>QRTGRSALAVLIRACYRLQQQLQRTRRALLHHSDAVLTSLHHVRMLL[2x];>IPAGIIPTGNVLSTIEVCIFFCIFDFFKQIRSDDNSLYSAQFDILLGTYCNTLNFVRFLELGLSVACICTKFPELAYVRDGVIQFEVQQPMIARDGPHPVDQPVHNYMVKRIHKRSLSAAFAIASEALSLLSNTYVAATEIDSSLRIRAIQQMARNLRTVSDSFERGTADQLLGVLLEKAPPLSLLSPINKFQPEGHLNRVARAALLSDLKRRVCADMFFMTRHAREPRLISAYLSDMVSCTQPSVMVSRITHTNTRGRQVDGVLVTTATLKRQLLQGILQIDDTAADVPVTYGEMVLQGTNLVTALVMGKAVRGMDDVARHLLDITDPNTLNIPSIPPQSNSDSTTAGLPVNARVPADLVIVGDKLVFLEALERRVYQATRVAYPLIGNIDITFIMPMGVFQANSMDRYTRHAGDFSTVSEQDPRQFPPQGIFFYNKDGILTQLTLRDAMGTICHSSLLDVEATLVALRQQHLDRQCYFGVYVAEGTEDTLDVQMGRFMETWADMMPHHPHWVNEHLTILQFIAPSNPRLRFELNPAFDFFVAPGDVDLPGPQRPPEAMPTVNATLRIINGNIPVPLCPISFRDCRGTQLGLGRHTMTPATIKAVKDTFEDRAYPTIFYMLEAVIHGNERNFCALLRLLTQCIRGYWEQSHRVAFVNNFHMLMYITTYLGNGELPEVCINIYRDLLQHVRALRQTITDFTIQGEGHNGETSEALNNILTDDTFIAPILWDCDALIYRDEAARDRLPAIRVSGRNGYQALHFVDMAGHNFQRRDNVLIHGRPVRGDTGQAIPITPHHDREWGILSKIYYYIVIPAFSRGSCCTMGVRYDRLYPALQAVIVPEIPADEEAPTTPEDPRHPLHAHQLVPNSLNVYFHNAHLTVDGDALLTLQELMGDMAERTTAILVSSAPDAGAATATTRNMRIYDGALYHGLIMMAYQAYDETIATGTFFYPVPVNPLFACPEHLASLRGMTNARRVLAKMVPPIPPFLGANHHATIRQPVAYHVTHSKSDFNTLTYSLLGGYFKFTPISLTHQLRTGFHPGIAFTVVRQDRFATEQLLYAERASESYFVGQIQVHHHDAIGGVNFTLTQPRAHVDLGVGYTAVCATAALRCPLTDMGNTAQNLFFSRGGVPMLHDNVTESLRRITASGGRLNPTEPLPIFGGLRPATSAGIARGQASVCEFVAMPVSTDLQYFRTACNPRGRASGMLYMGDRDADIEAIMFDHTQSDVAYTDRATLNPWASQKHSYGDRLYNGTYNLTGASPIYSPCFKFFTPAEVNTNCNTLDRLLMEAKAVASQSSTDTEYQFKRPPGSTEMTQDPCGLFQEAYPPLCSSDAAMLRTAHAGETGADEVHLAQYLIRDASPLRGCLPL[5x];> AMPFEIEVLLPGELSPAETSALQKCEGKIITFSTLRHRASLVDIALSSYYINGAPPDTLSLLEAYRMRFAAVITRVIPGKLLAHAIGVGTPTPGLFIQNTSPVDLCNGDYICLLPPVYGSADSIRLDSVGLEIVFPLTIPQTLMREIIAKVVARAVEDLNLMFSINEGCLLILALIPRLLALLIPRLLALVTREAAQLIHPEAPMLMLPIYETISSWISTSSRLGDTLGTRAILRVCVFDGPSTVHPGDRTAVIQV;> AMPFEIEVLLPGEISPAETSALQKCEGKIITFSTLRHRASLVDIALSSYYINGAPPDTLSLLEAYRMRFAAVITRVIPGKLLAHAIGVGTPTPGLFIQNTSPVDLCNGDYICLLPPVFGSADEIRLDSVGLEIVFPLTIPQTLMREIIAKVVARAVERTAADVICYNGRRYELETNLQHRDGSDAAIRTLVLNLMFSINEGTTLILTLITRLLRFPIYEAISSWISTSSRLGDTLGTRAILRVCVFDGPSTVHPGDRTAVIQV;> FKSTTQLIQQVSLTDFFRPDIEHAGSTVLILRHPTDLPALARHRAPPGRQTERLAEAWGQLLEASRAYVTSLSFIAACRAEEYTDKQAAEANRTAIVSAYGCSRMGARLIRFSECLRAMVQCHVFPHRFISFFGSLLEYTIQDNLCNITAVAKGPQEAARTDKTSTRRVTANIPACVFWDVDKDLHLSADGLKHVFLVFVYTQRRQREGVRLHLALSQLNEQCFGRGIGFLLGARICMYAAYTLIGTIPSESVRYTRRMERFGGYNVPTIWLEGVVWGGTNTWNEC;> MNAHLANEVQYDLGHARVGPSSLVHVIISSECLAAAGIPLAALMRGRPGLGTAANFQVEIQTRAHATGDCTPWCTAFAAYVPADAVGELLAPVVPAHPGLLPRASSAGGLFVSLPVVCDAQGVYDPYAVAALRLAWGSGASCARVILFSYDELVPPNTRYAADSTRIMRVCRHLCRYVALLGAAAPPAAKEAAAHLSMGLGESASPRPQPLARPHAGAPADPPIVGASDPPISPEEQLTAPGGDTTAAQDVSIAQENEEILALVQRAVQDVTRRHPVRARTGRAACGVASGLRQGALVHQAVSGGAMGAADADAVLAGLEPPGGGRFVAPAP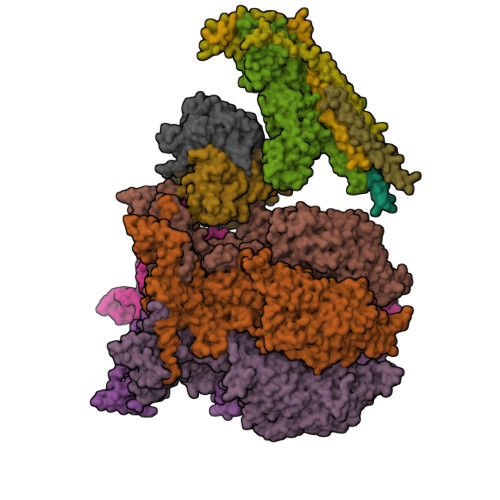HGPGGEDILNDVLTLTPGTAKPRSLVEWLDRGWEALAGGDRPDWLWSRRSISVVLRHHYGTKQRFVVVSYENSVAWGGRRARPPLLSSALATALTEACAAERVVRPHQLSPAGQAELLLRFPALEVPLRHPRPVLPPFDIAAEVAFTARIHLACLRALGQAIRAALQGGPRISQRLRYDFGPDQRAWLGEVTRRFPILLENLMRAVEGTAPDAFFHTAYALAVLAHLGGRGGRGRRVVPLGDDLPARFADSDGHYVFDYYSTSGDTLRLNNRPIAVAMDGDVSKREQSKCRFMEAVPSTAPRRVCEQYLPGESYAYLCLGFNRRLCGIVVFPGGFAFTINIAAYLSLSDPVARAAVLRFCRKVS;>[2x]MDPYCPFDALDVWEHRRFIVADSRNFITPEFPRDFWMSPVFNLPRETAAEQVVVLQAQRTAAAAALENAAMQAAELPVDIERRLRPIERNVHEI5-cyclopropyl-6-(3-methylimidazo[4,5-c]pyridin-7-yl)-3-[[3-methyl-1-[2,2,2-tris(fluoranyl)ethyl]pyrazol-4-yl]amino]pyrazine-2-carboxamide | C21 H20 F3 N9 O | 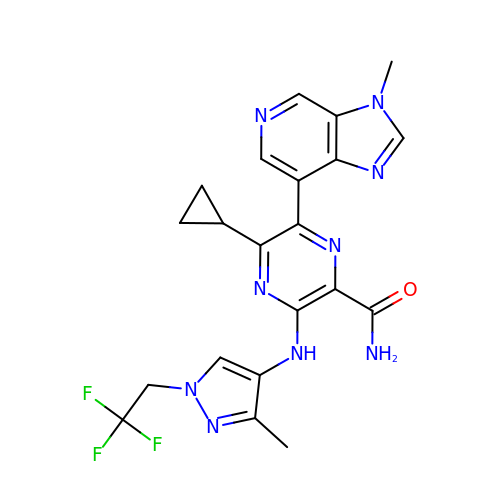YLGMPWWMPCGYBF-UHFFFAOYSA-N>ADGKILHNQNVNSWGPITVTPTTDGGETRFDGQIIVQMENDPVVAKAAANLAGKHAESSVVVQLDSDGNYRVVYGDPSKLDGKLRWQLV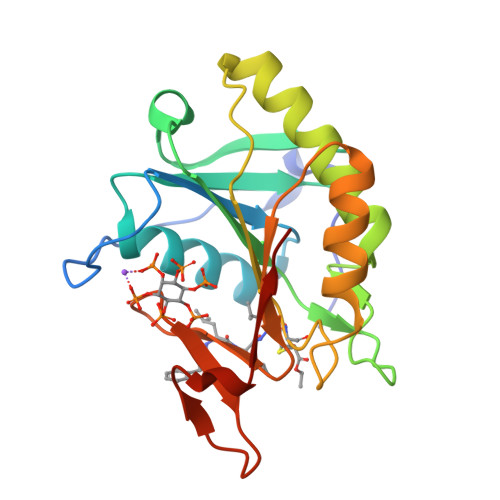GHGRDHSETNNTRLSGYSADELAVKLAKFQQSFNQAENINNKPDHISIVGCSLVSDDKQKGFGHQFINAMDANGLRVDVSVRSSELAVDEAGRKHTKDANGDWVQKAENNKVSLSWDAQG[4x]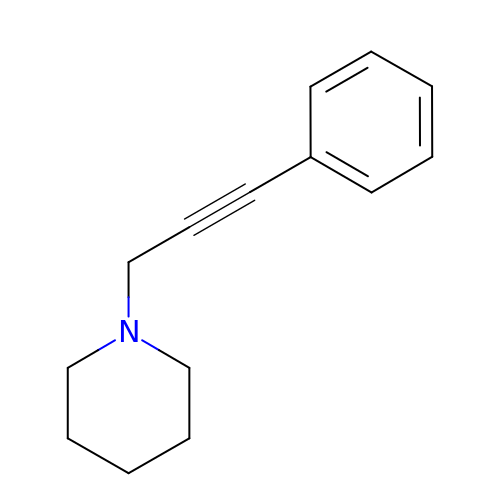1-(3-phenylprop-2-yn-1-yl)piperidine | C14 H17 N | PJMAQEATSLLDCR-UHFFFAOYSA-N>[2x]GAMGIPQHQQKHALMAIKAVKRLKDARPFLQPVDPVALNIPLYFNFIKRPMDLQTIERKLNANAYETPEQITEDFNLMVENSAKFNGPTAVITQMGRNIQAAFEKHMLNMPAKD

The fungal Bromodomain and Extra‐Terminal (BET) protein Bdf1 is a potential antifungal target against invasive fungal infections. One attractive target is the fungal BET protein Bdf1, a global transcriptional regulator. BET proteins bind chromatin through their two bromodomains (BDs), BD1 and BD2, which specifically recognize histones acetylated on lysines. We show that Bdf1 is essential in C. glabrata, and that inactivation of both Bdf1 BDs induces lethality.

We adapted our HTRF assay to perform a high‐throughput (HT) screen of small molecule inhibitors selective for CgBdf1 BDs over human BET BDs. We repurchased and rescreened these compounds and subsequently tested the 12 most potent hits against CgBD1 and CgBD2 and the corresponding human Brd4 BDs. This revealed 4 non‐selective inhibitors active against all four BDs and 8 compounds selective for CgBD1. To better understand the different selectivities of these compounds, we determined BD co‐crystal structures for the non‐selective tetrahydropyridoindole 29 and the CgBD1‐selective methylpyrazole 63. Structural alignments reveal that the binding pockets of CgBD1 and of Brd4 BD1 and BD2 can all accommodate 29, explaining its poor selectivity. The structure of CgBD1 bound to 63 shows that the latter's pyrazole 2‐nitrogen forms direct and water‐mediated H bonds with Asn209 and Tyr166, respectively, while its carboxyamide nitrogen forms a H bond with the Pro151 carbonyl. The oxadiazole and two thiophen moieties pack against residue Met218 within a shallow groove defined by residues Lys147 and RPF‐shelf residue Arg150 on one side and Val214 and Ile215 on the other. Structural alignments predict a severe clash between these moieties and the (W/Y)PF‐shelf residue corresponding to Arg150 in the two Brd4 BDs and in CgBD2. These observations highlight the initial residue of the (W/Y/R)PF‐shelf as an important ligand selectivity determinant.All these viruses utilize TfR1 as their cell entry receptor, and the ability to utilize human-TfR1 (hTfR1) distinguishes them from non-pathogenic viral species. As a potential broadly reactive immunotherapy against NW pathogenic mammarenaviruses, we designed a TfR1 mimetic that blocks the GP1 receptor-binding sites. Thus, we based our apical-domain design on wwTfR1 instead of on hTfR1 to achieve high-affinity targeting of pathogenic arenaviruses. We introduced several modifications to the wwTfR1-apical domain to allow it to be produced as a stand-alone protein. These modifications included the elimination of a long loop (residues 301–326) from the apical domain and the mutation of several hydrophobic residues at the interface between the apical- and protease-like domains to increase hydrophilicity.

To verify the binding mode of sAD to GP1, we crystallized and solved the structure of GP1MACV in complex with sAD to 2.7 Å resolution. Crystals belonged to a tetragonal space group (P4322) with four copies of sAD/GP1MACV in the asymmetric unit. The designed sAD forms a complex with GP1MACV in a similar fashion to hTfR128, while maintaining the overall structure of the hTfR1-apical domain. Most of the important interactions that GP1MACV makes with hTfR1 are also formed with sAD, including the key interaction with Tyr211. We did observe some structural differences; however, the long loop that connects parallel strands βII-6 and βII-7 of sAD, which was mutated and shortened, changed its conformation compared with hTfR1. In the case of hTfR128, Glu294 from this loop forms a salt bridge with Lys169 of GP1MACV, and in the case of sAD an alternative salt bridge with Lys169 is formed with Glu340 from αII-2 instead. In the crystal structure of sAD/GP1MACV, we observed electron density for N-acetylglucosamine only at the Asn251 glycosylation site of sAD and not near Asn204. In the sAD/GP1MACV structure, Asn204 of sAD is in close proximity to GP1MACV, suggesting that an N-acetylglucosamine attached to this residue will sterically prevent the formation of a complex. We thus introduced an S206A mutation to the sAD portion of Arenacept (referred to as Arenacept-M1) to eliminate the N-X-T/S glycosylation motif.

>[4x]KIQVKCSAPNSVTITNASGGLYLVEYPEGYVAYSKATEVTGKLVHANFGTKKDFEDLDYAVNGSIVIVRAGKITIAEKVANAQSFNAIGVLIYKDRTKYPISRADEPLQGHSGLPSIPVQTISREAAEKLFQNMERDCPRSWNTDSSCKLELLQNRNVKLTVNNCLKEGTSGHHHHHH;>[4x]SNELPSLCMLNNSFYYMRGGVNTFLIRVSDISVLMKEYDVSIYEPEDLGNCLNKSDSSWAIHWFSNALGHDWLMDPPMLCRNKTKKEGSNIQFNISKADDARVYGKKIRNGMRHLFRGFHDPCEEGKVCYLTINQCGDPSSFDYCGVNHLSKCQFDHVNTGSHHHHHH>QDPLSCYDNFGNRDVAACARFIDDFCDTLTPNIYRPRDNGQRCYVVNGHKCDFTVFNTNNGGSPIRASTPNCKTVLRAAANRCPTGGRGKINPSAPFLFAIDPNDGDCSTDF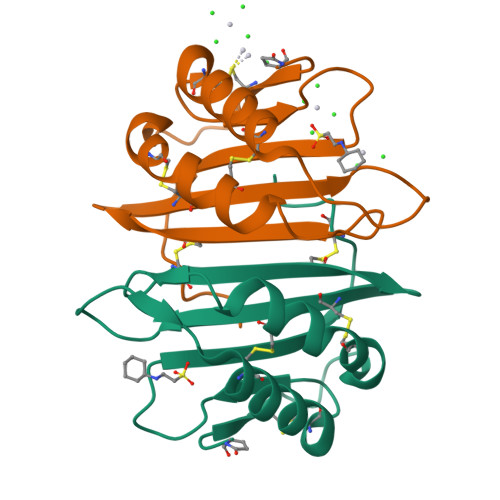[2x]>MEFWGVEVKNGKPLHLDPGLDRLVHISQVALGESKNNVTEPIQLYVTVGSDKLLIGTLSHEKFPQ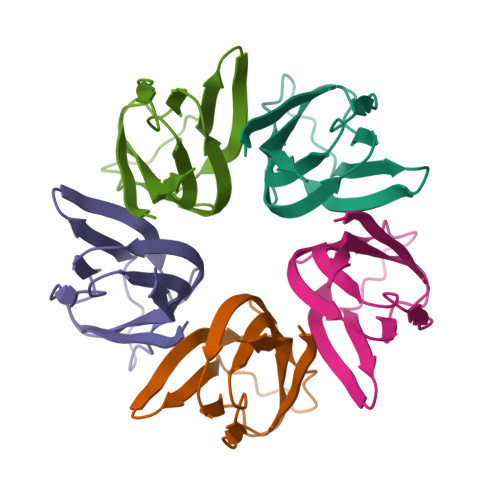LSTEIVLERNFALSHTWKNGSVFFSGYKVDL[5x]>[2x]MTPISQTPGLLAEAMVDLGAIEHNVRVLREHAGHAQLMAVVKADGYGHGATRVAQTALGAGAAELGVATVDEALALRADGITAPVLAWLHPPGID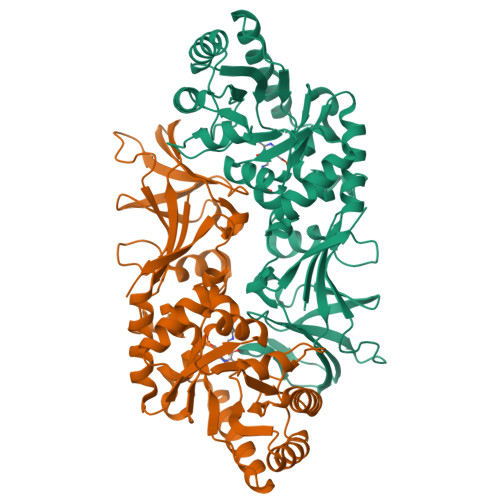FGPALLADVQVAVSSLRQLDELLHAVRRTGRTATVTVKVDTGLNRNGVGPAQFPAMLTALRQAMAEDAVRLRGLMSHMVYADKPDDSINDVQAQRFTAFLAQAREQGVRFEVAHLSNSSATMARPDLTFDLVRPGIAVYGLSPVPALGDMGLVPAMTVKCAVALVKSIRAGEGVSYGHTWIAPRDTNLALLPIGYADGVFRSLGGRLEVLINGRRCPGVGRICMDQFMVDLGPGPLDVAEGDEAILFGPGIRGEPTAQDWADLVGTIHYEVVTSPRGRITRTYREAENR> MNLTVNGKPSTVDGAESLNVTELLSALKVAQAEYVTVELNGEVLEREAFDATTVKDGDAV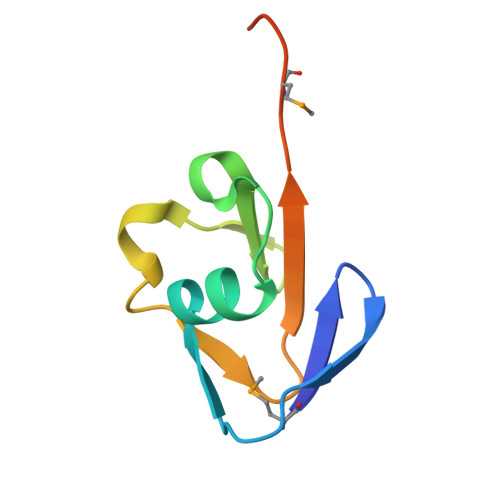EFLYFMGGGKLEHHHHHH> 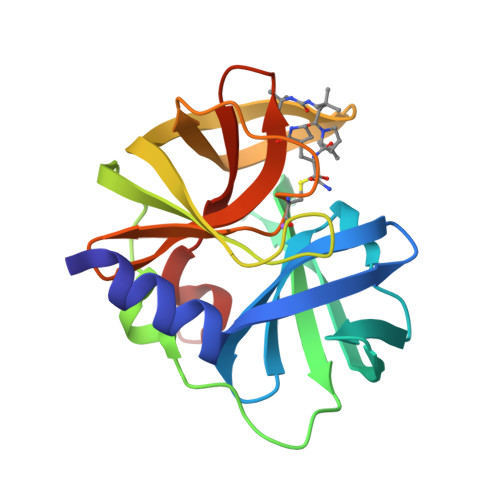PSLDFALSLLRRNIRQVQTDQGHFTMLGVRDHLAVLPRHSQPGKTIWVEHKLVRIVDAVELVDEQGVNLELTLVTLDTNEKFRDITRFIPETISPASDATLVINTEHMPSMFVPVGDVVQYGFLNLSGKPTHRTMMYNFPTKAGQCGGVVTAVGKVIGIHIGGNGRQGFCAALKRGYFCSEQ>MTGKGKDIIYGNECRNELLKGILTVSDVVKLTLGPRGRNVLLEKEYGSPLIINDGVTIAKQISLKDRKKNNGVKLMQESTQISNDKAGDGTSSTALMTATITKKGIEQVNRNHNPIPIQRGIQLASKMIIEKIKSLSTPIKTYKDILNIATIASN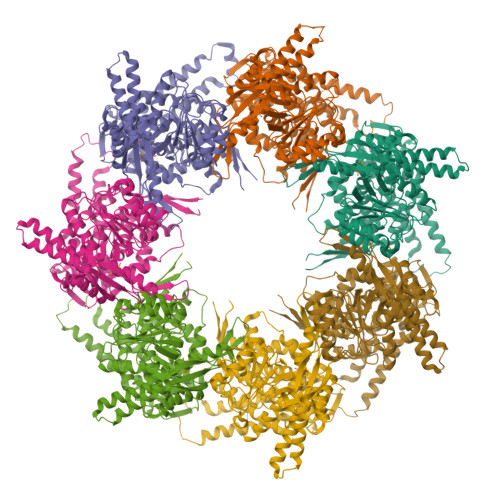NDVHMGQIIANAYDKLGKNAAIILDDNADINDKLEFTEGYNFDRGIINPYLLYNENKDYIEYSQVSTLITDQNIDNIQSILPILEIFAKNKQPLCIIADDFSNEVLQTLIINKLKGAIKVVPIRAPSFGDRRKDYLKDLCIVTNSKYISADVGLDLNNLHNQMSSFDNNYLSLLGSANTLIVKKDRTSLITKEEYKKEIDERINVLKKEYEETTSKYDKEKLNERIAALSGGIAKILIGGNSETEQKERKFKYEAATNAVKSAIDIGYVPGGGVTYLEIIKSNFIQEIHKKIEEDLQISSNNDEKKYLELIGNLESEMELQKMGANIVVSSLDVITKQIADNAGVNGDNVVKIILNSKDKYGFGYDVNTNKFVNMVEKGIIDSTNVIISVIKNSCSIASMVLTTECMMVDHEK[7x]> MTPEECRAQYRLMLKEAMDAYHQLNLGGSVRVVVDQNSERVEYTAANRQSLWAYIVRLQNAINSD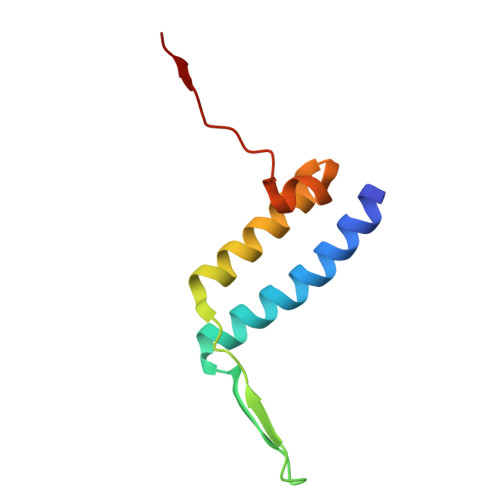NPCAAFMGLPSSPAGFLFP> AVDRDTAKNSSPIAGNIE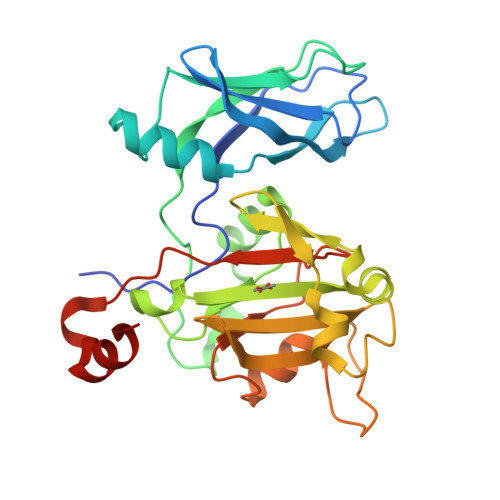YTISTPGSNYAVGDKITVKYVSDDIETEGKITEVDADGKIKKINIPTAKIIAKAKEVGEYPTLGSNWTAEISSSSSGLAAVITLGKIITDSGILLAEIENAEAAMTAVDFQANLKKYGIPGVVALYPGELGDKIEIEIVSKADYAKGASALLPIYPGGGTRASTAKAVFGYGPQTDSQYAIIVRRNDAIVQSVVLSTKRGGKDIYDSNIYIDDFFAKGGSEYIFATAQNWPEGFSGILTLSGGLSSNAEVTAGDLMEAWDFFADR> SPVVVVTGASRGIGKAIALSLGKAGCKVLVNYARSAKAAEEVSKQIEAYGGQAITFGGDVSKEADVEAMMKTAIDAWGTIDVVVNNAGITRDTLLIRMKKSQWDEVIDLNLTGVFLCTQAATKIMMKKRKGRIINIASVVGLIGNIGQANYAAAKAGVIGFSKTAAREGASRNINVNVVCPGFIASDMTAKLGEDME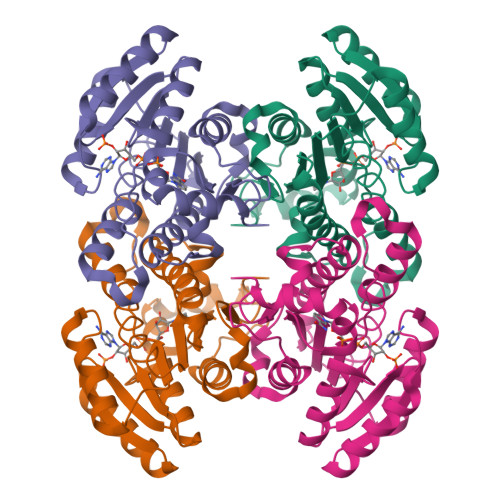KKILGTIPLGRTGQPENVAGLVEFLALSPAASYITGQAFTIDGGIAI> ETGETPPRFTRTPVDQTGVSGGVASFICQATGDPRPKIVWNKKGKKVSNQRFEVIE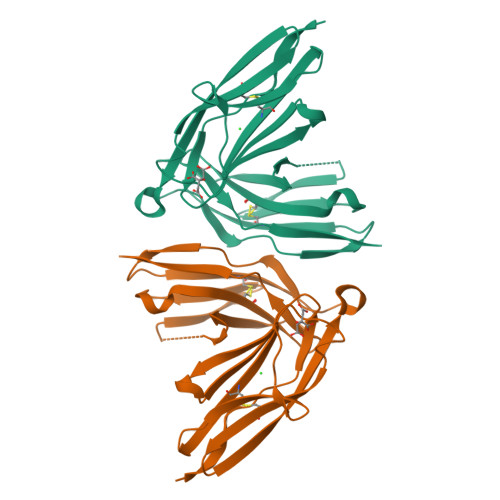FDDGSGSVLRIQPLRTPRDEAIYECVASNNVGEISVSTRLTVLREDQIPRGFPTIDMGPQLKVVERTRTATMLCAASGNPDPEITWFKDFLPVDTSNNNGRIKQLRSESIGALQIEQSEESDQGKYECVATNSAGTRYSAPANLYVRGTKHHHHHH> NLFQFARLIDAKQEAFSFFKYISYGCYCGWGGQGTPKDATDRCCFVHDCCYARVKGCNPKLVEYSYSYRTGKIVCGGD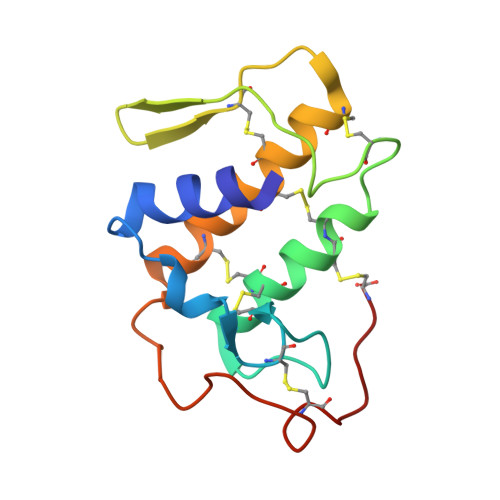DPCLRAVCECDRVAAICFRENMNTYDKKYMLYSIFDCKEESDQC> ALSARTQSSTGTHGGYY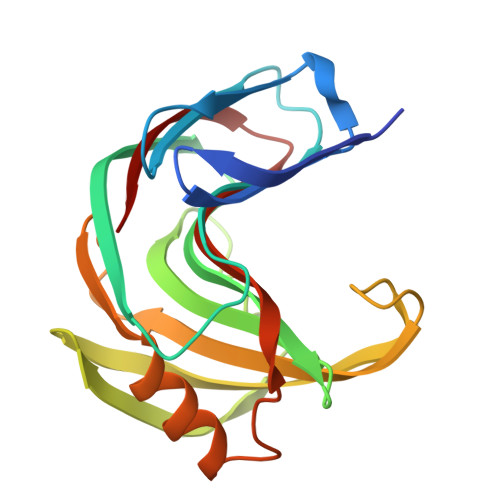YSFWTDNPNTVTYTNQNAGQFSVSWSGNQGNFVGGKGWNPGAARTIKYSGTYNPNGNSYLAVYGWTRNPLIEYYIVENFGTYNPSSGATAAGEVTVDGSVYDIYTSTRTNAPSIEGTRTFQQYWSVRRNKRSSGSVNTGAHFNAWSNVGLALGSHDYQILAVEGYYSSGSATMTVS> MQFSKMHGLGNDFVVVDGVTQNVFFTPETIRRLANRHCGIGFDQLLIVEAPYDPELDFHYRIFNADGSEVSQCGNGARCFARFVTLKGLTNKKDISVSTQKGNMVLTVKDDNQIRVNMGEPIWEPAKIPFTANKFEKNYILRTDIQTVLCGAVSMGNPHCVVQVDDIQTAN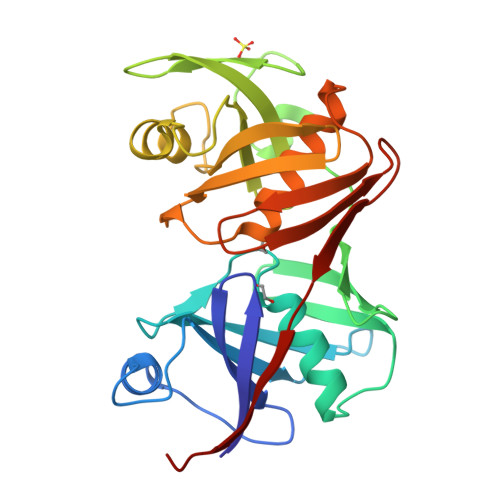VEQLGPLLESHERFPERVNAGFMQIINKEHIKLRVYERGAGETQASGSGACAAVAVGIMQGLLNNNVQVDLPGGSLMIEWNGVGHPLYMTGEATHIYDGFITL The T6SS of Pseudomonas aeruginosa transports two lytic enzymes, Tse1 and Tse3, to degrade cell-wall peptidoglycan in the periplasm of rival bacteria that are competing for niches via amidase and muramidase activities, respectively. Two cognate immunity proteins, Tsi1 and Tsi3, are produced by the bacterium to inactivate the two antibacterial effectors, thereby protecting its siblings from self-intoxication. Among the delivered proteins, Tse1 and Tse3 are biochemically characterized as lytic antibacterial enzymes that degrade the peptidoglycan of recipient bacterial cells, thereby causing rapid cell lysis of competing bacteria in the environment. It is now known that Tse1 functions as a peptidoglycan amidase with specificity towards γ-d-glutamyl-meso-2,6-diamino­pimelic acid (d-Glu-mDAP), while Tse3 functions as a mur­amidase that hydrolyzes the β-1,4-linkage between MurNAc and GlcNAc. Since the peptidoglycan of P. aeruginosa itself is not inherently resistant to Tse1 or Tse3, to protect its siblings the bacterium synthesizes two immunity proteins, Tsi1 and Tsi3, in the periplasmic compartment to specifically bind the cognate virulence effectors delivered from neighbouring cells, thereby resisting self-intoxication.

The crystal structure of the Tse3–Tsi3 complex was solved by SAD phasing using selenomethionine-substituted protein and was refined at 1.9 Å resolution. The two protein molecules form a compact complex with overall dimensions of 60 × 58 × 93 Å, and the molar ratio of Tse3 and Tsi3 agrees well with the 1:1 stoichiometry observed in solution. The results reveal that Tse3 contains a C-terminal catalytic domain that adopts a soluble lytic transglycosylase (SLT) fold in which three calcium-binding sites were surprisingly observed close to the catalytic Glu residue. The refined structure at 1.9 Å resolution also unexpectedly shows three calcium-binding sites in Tse3, one resembling the EF-hand motif and the other two being non-EF-hand sites close to the catalytic Glu residue. The involvement of these two key catalytic residues in Ca2+ binding is astonishing and impressive, as calcium-binding sites so close to the active centre have never been observed in previously characterized lysozymes and lytic transglycosylases. Tsi3 comprises a single domain showing a β-sandwich architecture that is reminiscent of the immunoglobulin fold. Three loops of Tsi3 insert deeply into the groove of Tse3 and completely occlude its active site, which forms the structural basis of Tse3 inactivation. As a result, the adjacent Ca2+-binding sites (Ca1 and Ca2) harboured locally in this region are significantly stabilized, and Glu126 is directly involved in Ca2+ coordination as a ligating residue for Ca2.

> MTATSDLIESLISYSWDDWQVTRQEARRVIAAIRNDNVPDATIAALDKSGSLIKLFQRVGPPELARSLIASIAGRTTMQRYQARNALIRSLINNPLGTQTDNWIYFPTITFFDICADLADAAGRLGFAAAGATGVASQAIQGPFSGVGATGVNPTDLPSIAFGDQLKLLNKDPATVTKYSNPLGDLGAYLSQLSPQDKLNQAQTLVGQPISTLFPDAYPGNPPSRAKVMSAAARKYDLTPQLIGAIILAEQRDQTRDEDAKDYQAAVSIKSANTSIGLGQVVVSTAIKYELFTDLLGQPVRRGLSRKAVATLLASDEFNIFATARYIRYVANLASQQDLRKLPKTRGAFPSIDLRAYAGNPRNWPRDNVRALASEYTSRPWDDNLSPGWPMFVDDAYATFLDPGMRFPLEHHHHHH;> MKTVALILASLALLACTAESGVDFDKTLTHPNGLVVERPVGFDARRSAEGFRFDEGGKLRNPRQLEVQRQDAPPPPDLASRRLGDGEARYKVEEDDGGSAGSEYRLWAAKPAGARWIVVSASEQSEDGEPTFALAWALLERARLQLEHHHHHH>[3x]MMR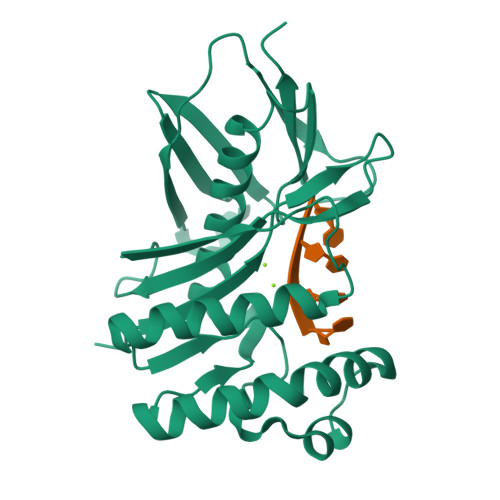IVAADTGGAVLDETFEPIGLIATVAVLVEKPYRSAKEVMVKYANPYDYDLTGRQAIRDEVLLAIELARKVKPDVIHLDSTLGGIELRKLDEPTIDALGISDKGKEVWKELSKDLQPLARKFWEETNIEIVAIGKSSVPVRIAEIYAGIYSAKWGIENVEKEGHLIIGLPRYMEVNIKDGKIIGRSLDPREGGLYGSAEVSVPEGVKWEIYPNPVARRFMIFEIFSKR>[8x]SSSKISRETLHQLIENKLCQAGLKREHAATVAEVLVYADARGIHSHGAVRVEYYAERISKGGTNREPEFRLEETGPCSAILHADNAAGQVAAKMGMEHAIKTAQQNGVAVVGISRMGHSGAISYFVQQAARAGFIGISMCQSDPMVVPFGGAEIYYGTNPLAFA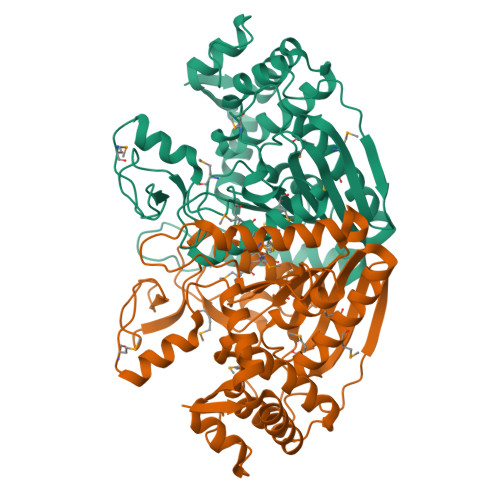APGEGDEILTFDMATTVQAWGKVLDARSRNMSIPDTWAVDKNGVPTTDPFAVHALLPAAGPKGYGLMMMIDVLSGVLLGLPFGRQVSSMYDDLHAGRNLGQLHIVINPNFFSSSELFRQHLSQTMRELNAITPAPGFNQVYYPGQDQDIKQRKAAVEGIEIVDDIYQYLISDALYNTSYETKNPFAQ>[2x]GGTDINKLIEEGKKHYLPKTYTFDNGKIIIKAGDKVEESKIQKLYWASKEVKSQFHRIIGNDKPLEVGNADDILTIVIYNNPEEYKLNKTLYGYSVDNGGIYIEGIGTFFTYERTPQESIYSLEELFRHEFTHYLQGRYLIPGLFNKGDFYKGNNGRITWFEEGSAEFFAGSTRTSVLPRKSMVGGLSKNPKERFNADKLLHSKYSDGWDFYKYGYAFSDYMYNNNKKLFSDLVSTMKNNDVKGYEALIEESSKDSKINKDYEYHMENLVNNYDNYTIPLVSDDYMKQYDNKSLHEIKSDIEKAMDVKNSQITKESSQYFDTYNLKATYTLSSNKGEISNWNYMNNKINEALNKLDNLSWGGYKTVTAYFSNPRLNSNNEVVYDIVFHGLLSHN

Clostridial collagenases are among the most efficient enzymes to degrade by far the most predominant protein in the biosphere. Clostridia employ collagenases for nutrition (e.g. saprophytic strains) and host colonization (1–3). They are large multidomain proteins of ∼115 kDa belonging to the gluzincin superfamily of metalloproteases. Here we present the crystal structures of the peptidase domains of ColH and ColT and the collagenase unit of ColG in the presence and absence of the peptidic inhibitor isoamylphosphonyl-Gly-Pro-Ala bound to the active site.

As described analogously for ColG, inhibitor binding induced a 2-Å contraction of these segments in ColT. This conformational breathing emphasizes the hingelike active site topology in clostridial collagenases. Although all peptidases adopted an open conformation in the unliganded apo-form and a more compact conformation in the complexed state, this breathing movement was most pronounced in ColG and least pronounced in ColH. Notably, the peptidase domain of ColG from C. histolyticum showed a higher structural similarity to ColT from C. tetani than to ColH from C. histolyticum. This structural relation is in particular evidenced by the extent of peptidase half-domain motions accompanying inhibitor binding and may, on a functional level, reflect the substrate specificities of the three homologous collagenases. The interaction areas between the inhibitor isoamylphosphonyl-GPA with the individual enzymes is largest in ColH (256 Å2) > ColT (248 Å2) > ColG (220 Å2), as calculated using the PISA server. The characteristic HEXXH consensus sequence is located on the central helix; the third proteinaceous zinc ligand is a glutamate located 28 residues (ColG and ColH) or 30 residues (ColT) downstream on the neighboring gluzincin helix. The spatial arrangement of the zinc ligands is identical in all three peptidases, notwithstanding the difference in sequential separation.> GSGYSSEKIPVTGSGFVAKDDSLRTFFDAMALQLKEPVIVSKMAARKKITGNFEFHDPNALLEKLSLQLGLIWYFDGQAIYIY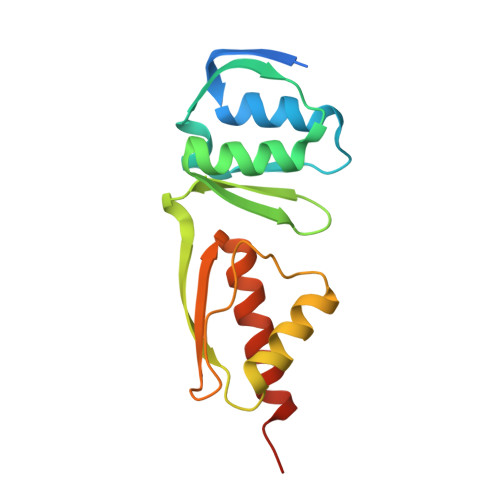DASEMRNAVVSLRNVSLNEFNNFLKRSGLYNKNYPLRGDNRKGTFYVSGPPVYVDMVVNAATMMDKQNDGIELGRQ>[2x]FDRNVPRICGVCG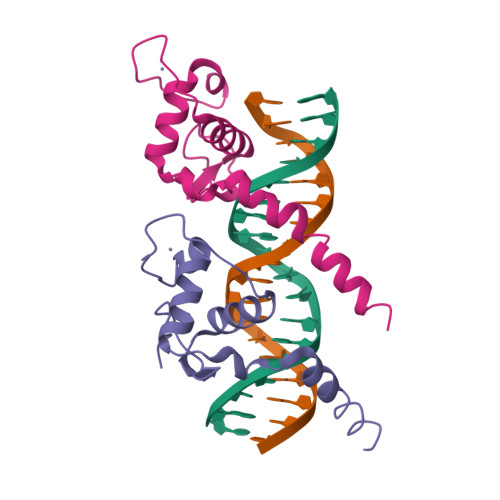DRATGFHFNAMTCEGCKGFFRRSMKRKALFTCPFNGDCRITKDNRRHCQACRLKRCVDIGMMKEFILTDEEVQRKREMILKRKEEEALKDSLRPKLS2-(1-hydroxy-6-((2-(4-methyl-3-oxopiperazin-1-yl)-2-oxoethyl)carbamoyl)-1,3-dihydrobenzo[c][1,2]oxaborol-3-yl)acetic acid | C17 H20 B N3 O7 | 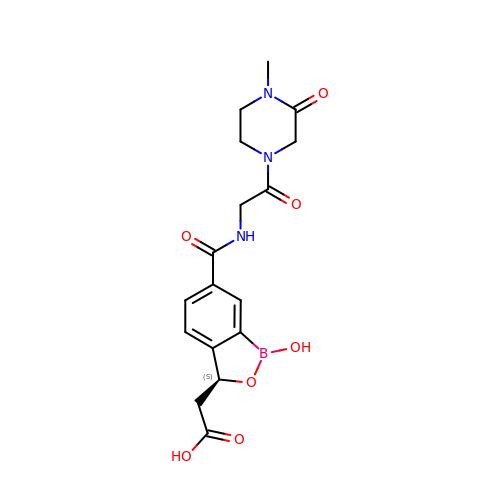WBGRQHYZWFAHOW-ZDUSSCGKSA-N>[2x]MASEALTMIVNLLRSQRPLQEPTVEQMRAGLEAMAQM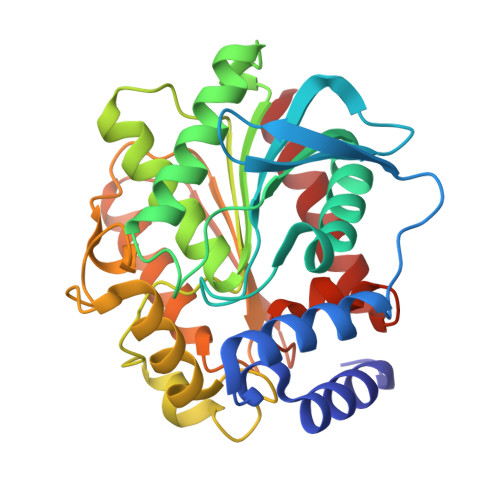SPLPADVELTTVDAGGVPGAWVRVPESDPDRVVLYLHGGGYVIGSIRTHRDLAQRIARAARCRVLLIDYRLAPEHPHPAAVEDSTRAYRWLLETGSDPKRMAIAGDAAGGGLTVATLVALRDAGVPLPAAAVCLSPWVDLEGIGESMTTKAAVDPMVQREPLLRMASMYLAGQDPRTPLAAPLYADLRGLPPLLIQVGTAETLLDDSVRLAERARAAGVQVTLEPWEDMIHVWQAFAAMLPEGQQAIERIGEFLRQHWQ> IIDGYKCKEGSHPWQVALLKGNQLHCGGVLVDKYWVLTAAHCKMGQYQVQLGSDKIGDQSAQKIKATKSFRHPGYSTKTHVNDIMLVRLDEPVKMSSKVEAVQLPEHCEPPGTSCTVSGWGTTTSPDVTFPSDLMCSDVKLISSRECKKVYKDLLGKTMLCAGIP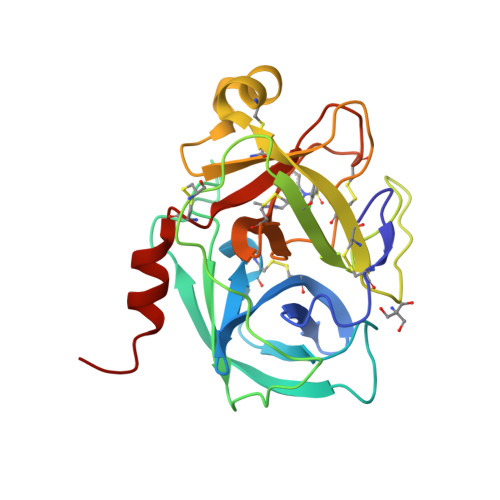DSKTNTCNGDSGGPLVCNDTLQGLVSWGTYPCGQPNDPGVYTQVCKYKRWVMETMKTHR Phylogenetically diverse bacteria can carry out chloramphenicol reduction, but only a single enzyme has been described that efficiently catalyzes this reaction, the NfsB nitroreductase from Haemophilus influenzae strain KW20. We found that expression of H. influenzae and Neisseria spp. nfsB genes, but not Pasteurella multocida nfsB, allows Escherichia coli to resist chloramphenicol by nitroreduction. Mass spectrometric analysis confirmed that purified H. influenzae and N. meningitides NfsB enzymes reduce chloramphenicol to amino-chloramphenicol, while kinetics analyses supported the hypothesis that chloramphenicol reduction is a secondary activity. Previous kinetic studies of nitroreductase catalysis revealed that reactions progress by a double-displacement (ping-pong) mechanism that appears to lack the gating steps necessary to impose specificity, explaining the substrate promiscuity of these enzymes.

Hi 12 NfsB showed both the fastest apparent maximum rate and, overall, significantly higher activity (>2-fold more active; q < 0.005) than Hi KW20 NfsB as measured by catalytic efficiency (kcat/Km). We also soaked an analog of chloramphenicol, 4-nitrophenol, into Hi 12 NfsB crystals and solved the resulting enzyme-substrate complex. Similarly, when Hi 12 NfsB contains 4-nitrophenol in its active site, Trp71 swings out, with movement potentially of the whole α3-to-α4 loop, to avoid a clash with the 4-nitrophenol NO2 group. This movement appears to be supported through an interaction with the Met74 side chain, in which the S (Sδ) of Met attracts the Trp71 aromatic ring through a long π-π interaction (7 to 10 Å). For structural changes specific to substrate binding (e.g., nitroaromatics), as opposed to coenzyme binding (e.g., NADPH), we focused on comparisons between the Hi 12 NfsB structure complexed with 4-nitrophenol, the Nm Z2491 structure complexed with nicotinic acid, and the previously published En. cloacae structures complexed with 4-nitrobenzoic acid or NAAD. The phenyl rings of nicotinic acid in the Nm Z2491 NfsB structure and 4-nitrobenzoic acid in the En. cloacae structure coincide with the niacin ring of NAAD in the other En. cloacae structure. The 4-nitrophenol molecule, complexed with Hi 12 NfsB, takes the same position, although rotated approximately 50° around its hydroxy oxygen. We have identified that the NfsB homolog from H. influenzae strain 12 exhibits the highest chloramphenicol reduction activity thus far, likely due to increased flexibility in the small loop between α3 and α4 in the active site.

>[2x]SNAMTQLTREQVLELFHQRSSTRYYDPAKKISDEDFECILECGRLSPSSVGSEPWKFLVIQNKTLREKMKSFSWGMMNQLDNCSHLVVILAKKNARYDSPFFEDVMVRKGLNAEQQQAALAKYKALQEEDMKLLESDRTLFDWCSKQTYIALANMLTGAAALGIDSCPIEGFHYDKMNECLAEEGLFDPKEYAVSVAATFGYRSRDIAKKSRKALDEVVRWVE> XDPPL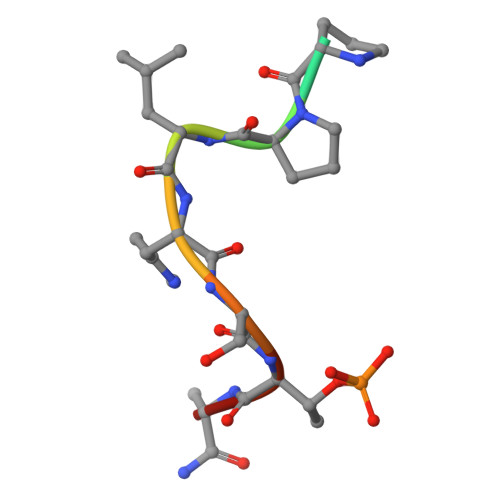HSTAX> ANPRENFLKCFSKHIPNNVANPKLVYTQHDQLYMSILNSTIQNLRFISDTTPKPLVIVTPSNNSHIQATILCSKKVGLQIRTRSGGHDAEGMSYISQVPFVVVDLRNMHSIKIDVHSQTAWVEAGATLGEVYYWINEKNENLSFPGGYCPTVGVGGHFSGGGYGALMRNYGLAADNIIDAHLVNVDGKVLDRKSMGEDLFWA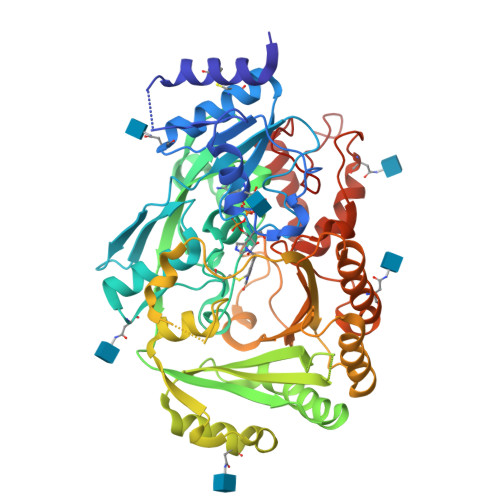IRGGGGENFGIIAAWKIKLVAVPSKSTIFSVKKNMEIHGLVKLFNKWQNIAYKYDKDLVLMTHFITKNITDNHGKNKTTVHGYFSSIFHGGVDSLVDLMNKSFPELGIKKTDCKEFSWIDTTIFYSGVVNFNTANFKKEILLDRSAGKKTAFSIKLDYVKKPIPETAMVKILEKLYEEDVGAGMYVLYPYGGIMEEISESAIPFPHRAGIMYELWYTASWEKQEDNEKHINWVRSVYNFTTPYVSQNPRLAYLNYRDLDLGKTNHASPNNYTQARIWGEKYFGKNFNRLVKVKTKVDPNNFFRNEQSIPPLPPHHH>MKETNSEEADSGLAFFRNMYDKYRDAFLSHLNEYSLEEEIKEHISKYYKLLFDYNCLGGKNNRGILVILIYEYVKNRDINSSEWEKAACLAWCIEILQAAFLVADDIMDKGEMRRNKYCWYLLKDVETKNAVNDVLLLYNSIYKLIEIYLRNESCYVDVIATFRDATLKTIIGQHLDTNIFSDKYSDAHREIDVNNINVPEQPVIDINMINFGVYKNIVIHKTAYYSFFLPIVCGMLLAGIAVDNLIYKKI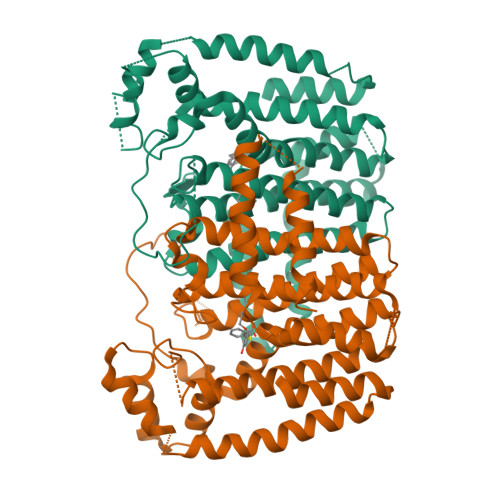EDISMLMGEYFQIHDDYLDIFGDSTKTGKVGSDIQNNKLTWPLIKTFELCSEPDKIKIVKNYGKNNLACVKVIDSLYEQYKIRKHYESYEKAQKAKILSAINELHHEGIEYVLKYLLEILFTGV[4x]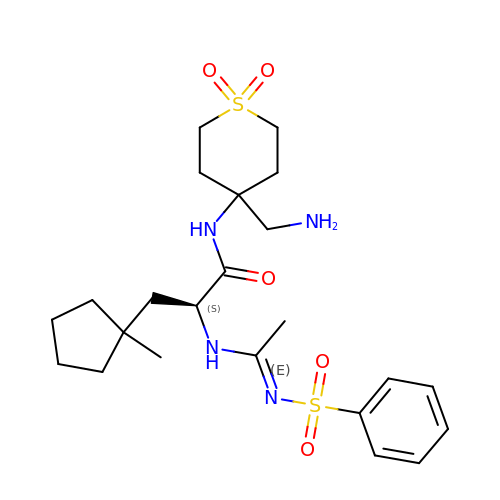N-[4-(AMINOMETHYL)-1,1-DIOXIDOTETRAHYDRO-2H-THIOPYRAN-4-YL]-3-(1-METHYLCYCLOPENTYL)-N~2~-[(1E)-N-(PHENYLSULFONYL)ETHANIMIDOYL]-L-ALANINAMIDE | C23 H36 N4 O5 S2 | HHATUZWPRPHWDY-FQEVSTJZSA-N> GPGSMVEQILAEFQLQEED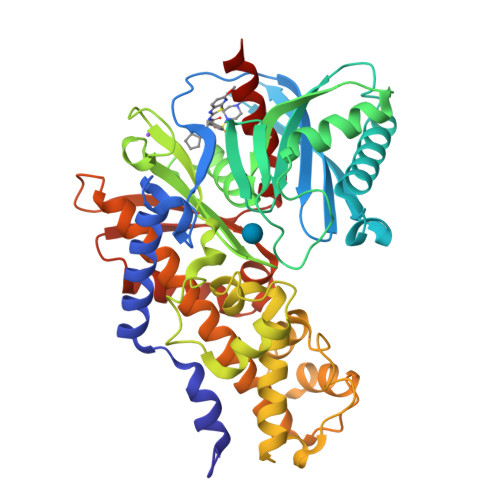LKKVMRRMQKEMDRGLRLETHEEASVKMLPTYVRSTPEGSEVGDFLSLDLGGTNFRVMLVKVGEGEEGQWSVKTKHQMYSIPEDAMTGTAEMLFDYISECISDFLDKHQMKHKKLPLGFTFSFPVRHEDIDKGILLNWTKGFKASGAEGNNVVGLLRDAIKRRGDFEMDVVAMVNDTVATMISCYYEDHQCEVGMIVGTGCNACYMEEMQNVELVEGDEGRMCVNTEWGAFGDSGELDEFLLEYDRLVDESSANPGQQLYEKLIGGKYMGELVRLVLLRLVDENLLFHGEASEQLRTRGAFETRFVSQVESDTGDRKQIYNILSTLGLRPSTTDCDIVRRACESVSTRAAHMCSAGLAGVINRMRESRSEDVMRITVGVDGSVYKLHPSFKERFHASVRRLTPSCEITFIESEEGSGRGAALVSAVACKKACMLGQ> MASEAIKGAVVGIDLGTTNSCVAVMEGKQAKVLENAEGARTTPSVVAFTADGERLVGMPAKRQAVTNPNNTFYATKRLIGWRYDDPEVQKDIKNVPFKIVRASNGDAWVEAHGKLYSPSQIGAFVLMKMKETAENYLGHTAKNAVITVPAYFNDSQRQATKDAGQISGLNVLRVINEPTAAALAYGLDKSEDKVIAVYDLGGGTFDISILEIQKGVFEVKSTNGDTFLGGEDFDQALLRHIVKEFKRETGVDLTKDNMALQRVREAAEKAKCELSSSVQTDINLPYLTMDSSGPKHLNMKLTRAQFEGIVTDLIRRTIAPCQKAMQDAEVSKSDIGEVILVGGMTRMPKVQQTVQDLFGRAPSKAVNPDEAVAIGAAIQGGVLAGDVTDVLLLDVTPLSLGIETLGG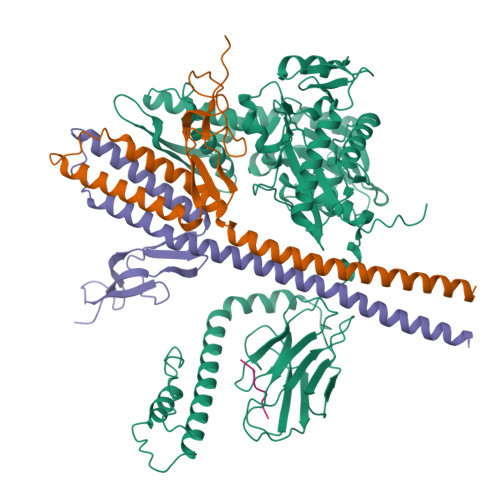VFTKLINRNTTIPTKKSQVFSTAADGQTQVEIKVCQGEREMAGDNKLLGQFTLIGIPPAPRGVPQIEVTFDIDANGIVHVSAKDKGTGREQQIVIQSSGGLSKDDIENMVKNAEKYAEEDRRKKERVEAVNMAEGIIHDTETKMEEFKDQLPADECNKLKEEISKMRELLARKDSETGENIRQAASS;>[2x]TLLEEKVKLEEQLKETVEKYKRALADTENLRQRSQKLVEEAKLYGIQAFCKDLLEVADVLEKATQCVPKEEIKDDNPHLKNLYEGLVMTEVQIQKVFTKHGLLKLNPVGAKFDPAEHEALFHTPVEGKEPGTVALVSKVGYKLHGRTLRPALVGVVKEASA;> VLLLDVT>MNPYERGPNPTDALLEARSGPFSVSEENVSRLSASGFGGGTIYYPRENNTYGAVAISPGYTGTEASIAWLGERIASHGFVVITIDTITTLDQPDSRAEQLNAALNHMINRASSTVRSRIDSSRLAVMGHAMGGGGSLRLASQRPDLKAAIPLTPWHLNKNWSSVTVPTLIIGADLDTIAPVATSAKPIYNSLPSSISKAYLELDGATHFAPNIPNKIIGKYSVAWLKRFVDNDTRYTQFLCPGPRDGLFGEVEEYRSTCPF[2x]

Cutinase is an esterase that belongs to the α/β-hydrolase superfamily and primarily hydrolyzes cutin from plants. Unlike lipases, cutinases lack the active site-covering lid structure such that the substrate-binding cleft is exposed and directly accessible from bulk solution. In addition, the substrate-binding site is more expansive in cutinases compared to esterases, benefiting the binding of bulkier macromolecules. In this work, we investigate the PBAT hydrolysis potency of cutinases and PET-degrading enzymes, and find that cutinases outcompete other reported enzymes.

We further constructed the inactive variant S170A to obtain a complex structure of BTa but failed to obtain any dataset that contains additional electron density that can be modeled with the ligand. We thus turned to a BTa-like compound MHET, which is composed of TPA and ethylene glycol linked via an ester bond. As a result, the structure of the S170A variant was determined in apo- and MHET-bound forms to 2.21 and 1.82 Å resolutions, respectively. The apo-form of S170A did not have an observable difference compared to TfCut-DM (Cα RMSD, 0.277 Å).> GSITQPTAINVIFPDPALANAIKIAAGKSNVTDTVTQADLDGITTLSAFGTGVTTIEGVQYLNNLIGLELKDNQITDLAPLKNLTKITELELSGNPLKNVSAIAGLQSIKTLDLTSTQITDVTPLAGLSNLQVLYLDLNQITNISPLAGLTNLQYLSIGNAQVSDLTPLANLSKLTTLKADDNKISDISPLASLPNLIEVHLKNNQISDVSPLANTSNLFIVTLTNQTITNQPVFYNNNLVVPNVVKGPSGAPIAPATISDNGTYASPNLTWNLTSFINNVSYTFN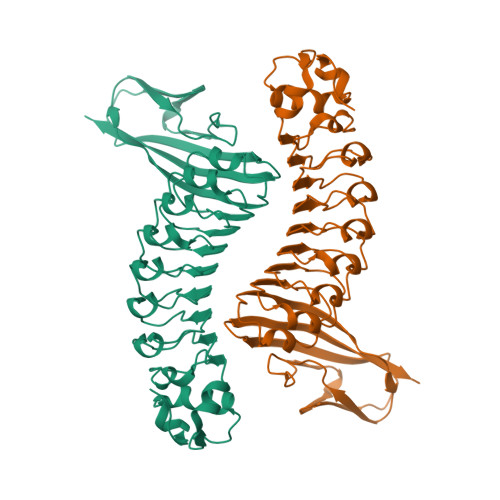QSVTFKNTTVPFSGTVTQPLTE> MHGRLKVKTSEEQAEAKRLEREQKLKLYQSATQAVFQKRQAGELDESVLELTSQILGANPDFATLWNCRREVLQHLETEKSPEESAALVKAELGFLESCLRVNPKSYGTWHHRCWLLSRLPEPNWARELELCARFLEADERNFHCW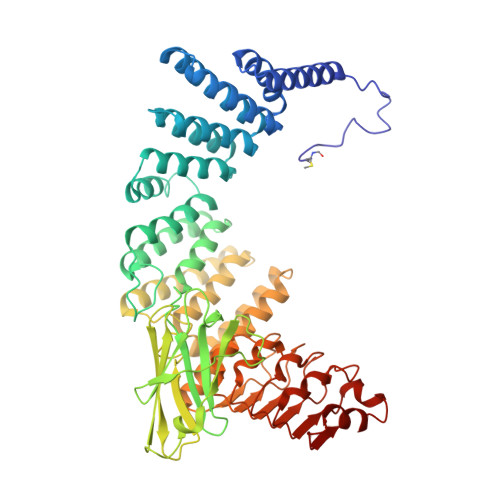DYRRFVAAQAAVAPAEELAFTDSLITRNFSNYSSWHYRSCLLPQLHPQPDSGPQGRLPENVLLKELELVQNAFFTDPNDQSAWFYHRWLLGRAEPHDVLCCVHVSREEACLSVCFSRPLTVGSRMGTLLLMVDEAPLSVEWRTPDGRNRPSHVWLCDLPAASLNDQLPQHTFRVIWTGSDSQKECVLLKDRPECWCRDSATDEQLFRCELSVEKSTVLQSELESCKELQELEPENKWCLLTIILLMRALDPLLYEKETLQYFSTLKAVDPMRAAYLDDLRSKFLLENSVLKMEYADVRVLHLAHKDLTVLCHLEQLLLVTHLDLSHNRLRALPPALAALRCLEVLQASDNALENVDGVANLPRLQELLLCNNRLQQSAAIQPLVSCPRLVLLNLQGNSLCQEEGIQERLAEMLPSVSSILT7-({[3-(3-fluorophenyl)propyl]amino}methyl)quinolin-2-amine | C19 H20 F 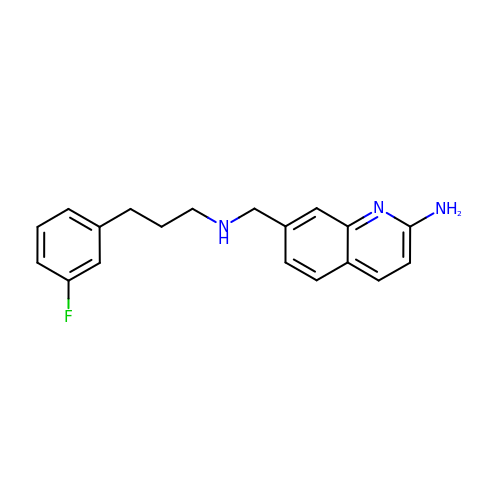N3 | QIPUHKWELQSESM-UHFFFAOYSA-N> NTKYNKEFLLYLAGFVDGDGSIIAQINPNASSKFKHRLRLTFYVTQKTQRRWFLDKLVDEIGVGYVRDSGSVSQYVLSEIAPLHNFLTQL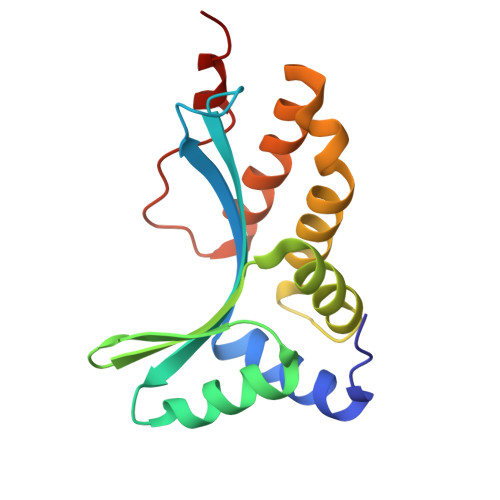QPFLKLKQKQANLVLKIIEQLPSAKASPAAFLEVCTWVDQIAALNDSATRKTTSETVAAVLD>GAMGSWNPKYDTRTLWTTPDTSPNCTIAQDKDSKLTLVLTKCGSQILANVSLIVVAGKYHIINNKTNPKIKSFTIKLLFNKNGVLLDNSNLGKAYWNFRSGNSNVSTAYEKAIGFMPNLVAYPKPSNSKKYARDIVYGTIYLGGKPDQPAVIKTTFNQETGCEYSITFNFSWSKTYENVEFETTSFTFSYIA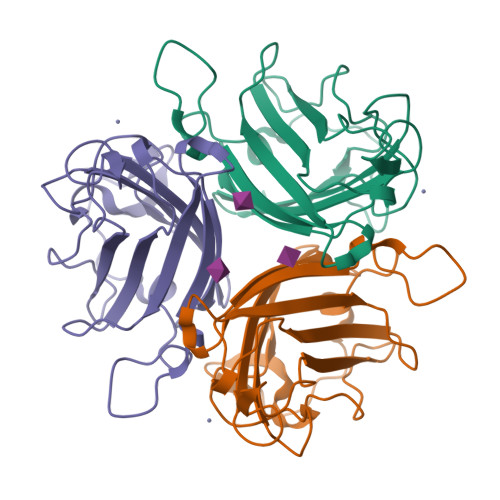QE[6x]3-[4-(2-{[4-(piperidin-4-yl)phenyl]amino}-6,7-dihydro-5H-pyrrolo[2,3-d]pyrimidin-4-yl)-1H-pyrazol-1-yl]propanenitrile 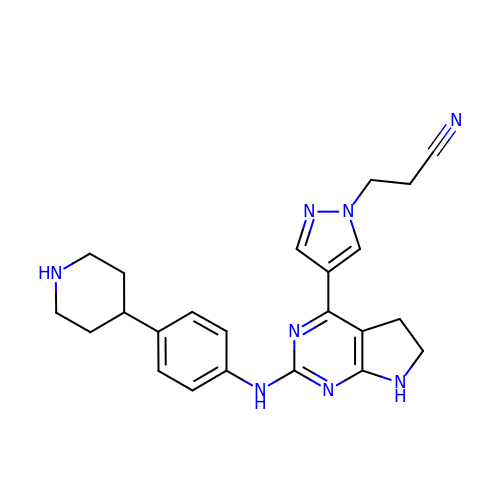| C23 H26 N8 | LADBWLAFXFHONI-UHFFFAOYSA-N(3-{4-[(4-cyclopropylphenyl)methoxy]-3-methoxyphenyl}azetidin-1-yl)(4-{[(2S)-2,3-dihydroxypropoxy]methyl}pyridin-2-yl)methanone 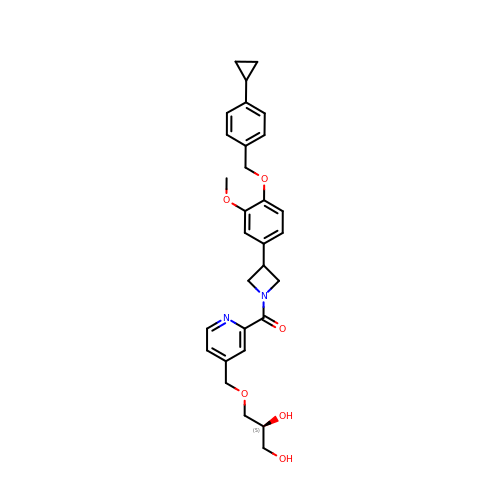| C30 H34 N2 O6 | LTTJGQBDGMNWHJ-SANMLTNESA-N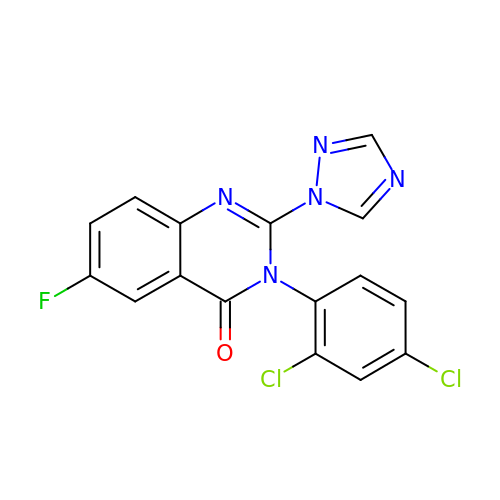3-(2,4-dichlorophenyl)-6-fluoranyl-2-(1,2,4-triazol-1-yl)quinazolin-4-one | C16 H8 Cl2 F N5 O | IJJVMEJXYNJXOJ-UHFFFAOYSA-N> MVIVPEGTQLDEKQHIVINNGAEPQSFDPHKTEGVPESNVAYQLLEGLVTSDSEGKLQPGAAESWE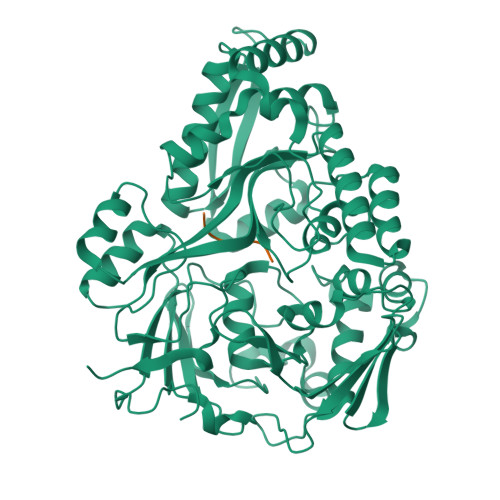NTPDFKTWTFHLRKDAKWSNGDPVTAHDFVFAWRRLVDPATAAPYASYLSYLQVENAQDIIDGKKKPAELGVEAKDDYTFVVHATNPVPYAVSLTTHQSLLPLPQKVVEKLGDAWVKKENYVGNGAYKLANHIINEKIEFERNPLYWNDKETVINSATFLAIENPSTDVARYRAGDLDMTSYGLPPEQFAKLKKELLGEVYVTRTLGTYSYELNNKKAPFDNVNIRKALNLSLDRNVITDKVLGQGQTPTYVFTPTYIEEGHLIQQPAYSKEPMAQRNEEAIKLLEEAGYSKANPLKFSILYNTNENHKKVAIAAASMWKANTKGLIDVKLENQEWKTYIDSRRAGRYDVARAGWHADYNQATTFGNYFLSNSSNNTAKYANPEYDKAMAESYAATDAEGRAKAYAKAEEILGKDYGIVPIFNYVNPRLVKPYVKGYSGKDPQDHIYLRNLYIIKHLEHHHHHH;> YLGANG> MGSNAPPPPTPHVVLVPFPGQGHVAPLMQLARLLHARGARVTFVYTQYNYRRLLRAKGEAAVRPPATSSARFRIEVIDDGLSLSVPQNDVGGLVDSLRKNCLHPFRALLRRLGQEVEGQDAPPVTCVVGDVVMTFAAAAA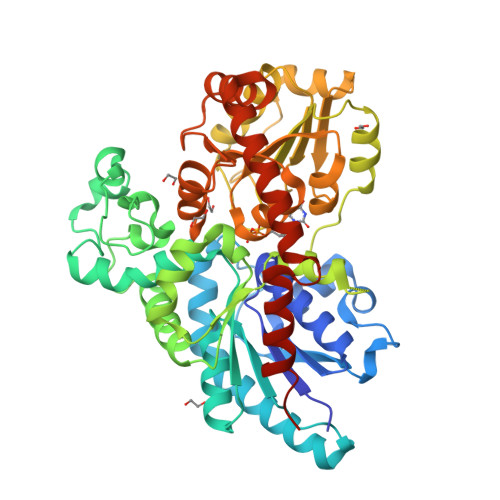REAGIPEVQFFTASACGLLGYLHYGELVERGLVPFRDASLLADDDYLDTPLEWVPGMSHMRLRDMPTFCRTTDPDDVMVSATLQQMESAAGSKALILNTLYELEKDVVDALAAFFPPIYTVGPLAEVIASSDSASAGLAAMDISIWQEDTRCLSWLDGKPAGSVVYVNFGSMAVMTAAQAREFALGLASCGSPFLWVKRPDVVEGEEVLLPEALLDEVARGRGLVVPWCPQAAVLKHAAVGLFVSHCGWNSLLEATAAGQPVLAWPCHGEQTTNCRQLCEVWGNGAQLPREVESGAVARLVREMMVGDLGKEKRAKAAEWKAAAEAAARKGGASWRNVERVVNDLLLVGGKQHHHHHH> MDLTNGGVSPAATSAPLDWTTFRRVFLIDDAWRPLMEPELANPLTAHLLAEYNRRCQTEEVLPPREDVFSWTRYCTPDEVRVVIIGQDPYHHPGQAHGLAFSVRANVPPPPSLRNVLAAVKNCYPEARMSGHGCLEKWARDGVLLLNTTLTVKRGAAASHSRIGWDRF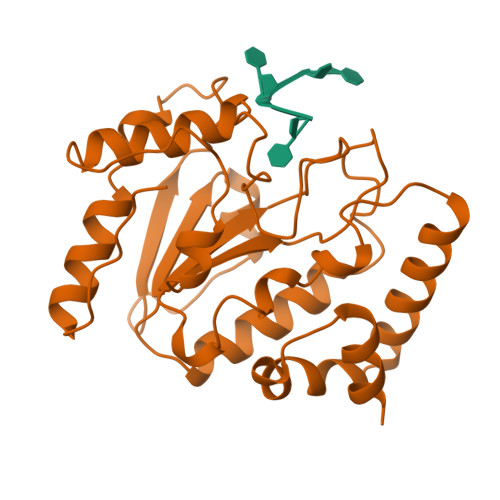VGGVIRRLAARRPGLVFMLWGTHAQNAIRPDPRVHCVLKFSHPSPLSKVPFGTCQHFLVANRYLETRSISPIDWSV> MTIGQKNTNIDPRFPHHHPRPQSFWEARAKALESLLI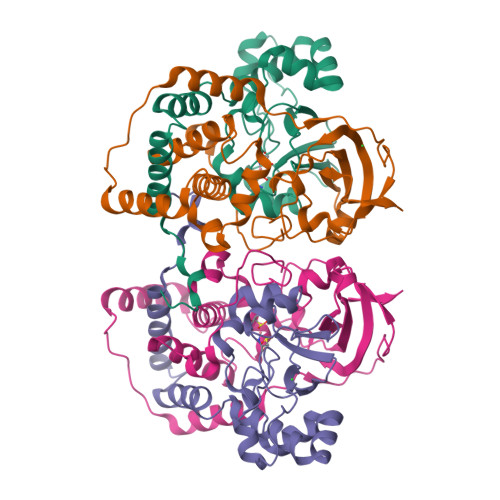EKGHLSSDAIERVIKHYEHELGPMNGAKVVAKAWTDPAFKQRLLEDSETVLRELGYYGLQGEHIRVVENTDTVHNVVVCTLCSCYPWPLLGLPPSWYKEPAYRARVVKEPRQVLKEFGLDLPDSVEIRVWDSSSEIRFMVLPQRPEGTEGMTEEELAKLVTRDSMIGVAKIEPPKVTVG;> MNGIHDVGGMDGFGKVMYVKEEEDIYFTHDWERLALGLVAGCMAQGLGMKAFDEFRIGIELMRPVDYLTSSYYGHWIATVAYNLVDTGVLDEKELDERTEVFSKKPDTKIPRREDPALVKLVEKALNDGLSPLREISASPRFKVGERIKTKNIHPTGHTRFPRYARDKYGVIDEVYGAHVFPDDAAHRKGENPQYLYRVRFEAEELWGYKQKDSVYIDLWESYMEPVSH>[6x]MQTASVPAGIAERRTRAWAPYIDAKLGFRNHWYPVRLSAEVAEASPVPVQLLGEKVLLNRVDGVVHAIADRCLHRG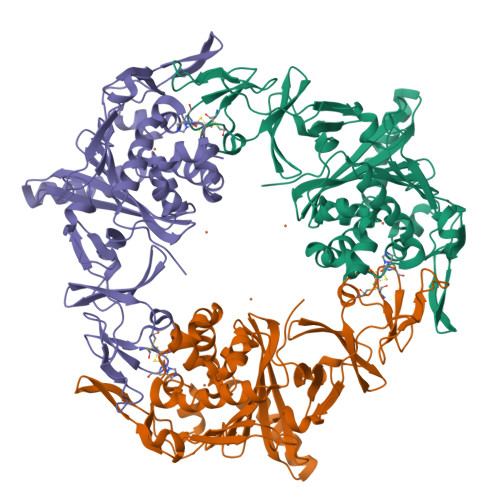VTLSDKVECYSKATISCWYHGWTYRWDNGKLVDILTNPTSVQIGRHALKTYPVREEKGLVFLFVGDQEPHDLAEDVPPGFLDADLAVHGQHRVVDANWRMGVENGFDAGHVFIHKSSILLDGNDIALPLGFAPGDPEQLTRSVTGEGAPKGVFDLLGEHSVPIFEATIEGQPAIQGHMGSKMVAISISVWLPGVLKVDPFPDPTLTQFEWYVPIDEGHHLYLQMLGRRVGSEEEARSFEAEFREKWVELALNGFNDDDILARRSMEPFYADDRGWREEVLFESDRAIIEWRRLASQYNRGIQTRDVRHHHHHH> MSHYHEQFLKQNPLAVLGV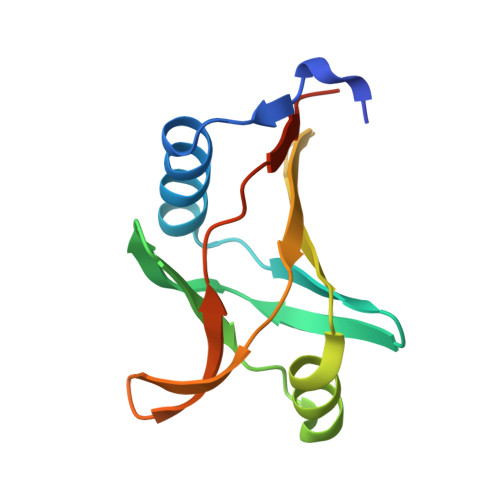LRDLHKAAIPLRLSWNGGQLISKLLAITPDKLVLDFGSQAEDNIAVLKAQHITITAETQGAKVEFTVEQLQQSEYLQLPAFITVPPPTLWFVLEHHHHHH> XE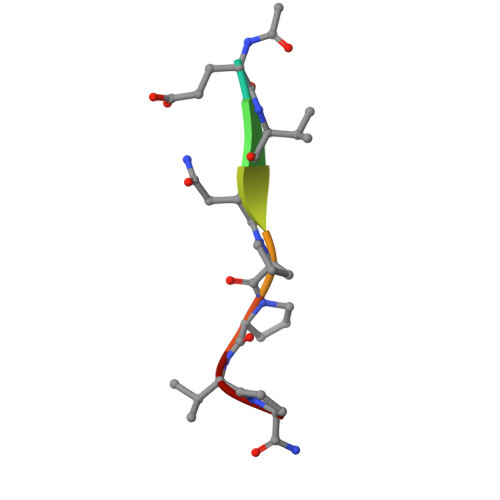VNPPVP5-FLUOROINDOLE PROPANOL PHOSPHATE | C11 H13 F N O4 P | 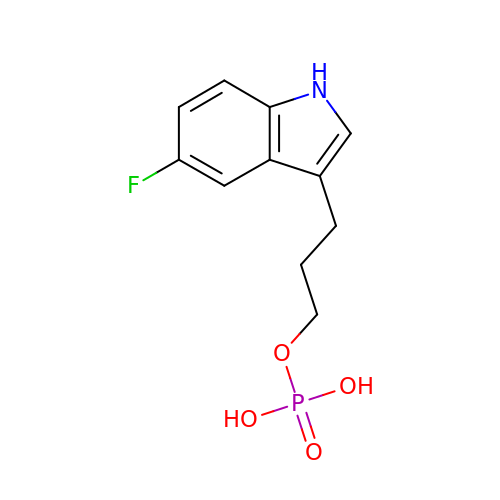YVYGGBFCYXRNKM-UHFFFAOYSA-N>MIREGDKVVLVDPRGKRYLITVSKRDFHTDLGILKLEEIIGRNFGEAIKSHKGHEFKILRPRIVDYLDKMKRGPQIVHPKDAALIVAYAGISPGDFIVEAGVGSGALTLFLANIVGPEGRVVSYEIREDFAKLAWENIKWAGFD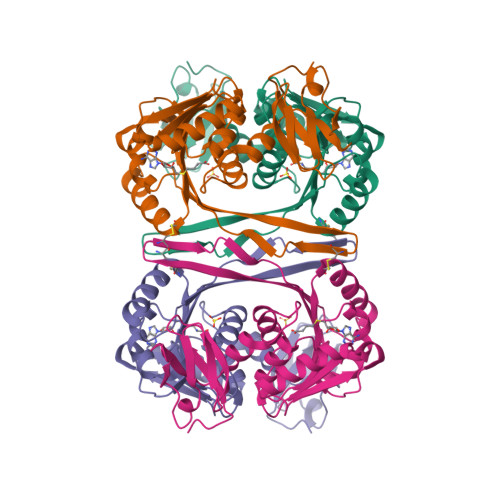DRVTIKLKDIYEGIEEENVDHVILDLPQPERVVEHAAKALKPGGFFVAYTPCSNQVMRLHEKLREFKDYFMKPRTINVLVFDQEVKKECMRPRTTALVHTGYITFARRI[4x]>[2x]GSHMNAAAEAEFNILLATDSYKVTHYKQYPPNTSKVYSYFECREKKTENSKVRKVKYEETVFYGLQYILNKYLKGKVVTKEKIQEAKEVYREHFQDDVFNERGWNYILEKYDGHLPIEVKAVPEGSVIPRGNVLFTVENTDPECYWLT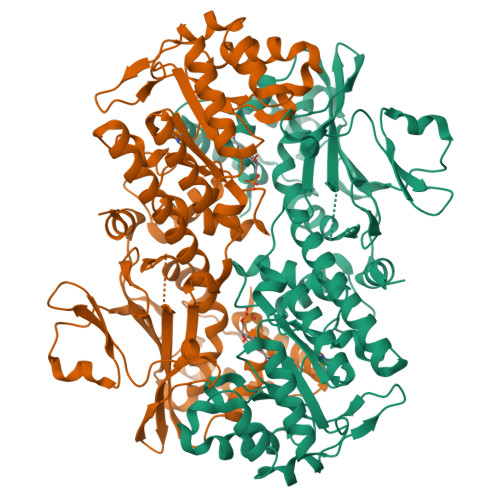NWIETILVQSWYPITVATNSREQKKILAKYLLETSGNLDGLEYKLHDFGYRGVSSQETAGIGASAHLVNFKGTDTVAGIALIKKYYGTKDPVPGYSVPAAEHSTITAWGKDHEKDAFEHIVTQFSSVPVSVVSDSYDIYNACEKIWGEDLRHLIVSRSTEAPLIIRPDSGNPLDTVLKVLDILGKKFPVTENSKGYKLLPPYLRVIQGDGVDINTLQEIVEGMKQKKWSIENVSFGSGGALLQKLTRDLLNCSFKCSYVVTNGLGVNVFKDPVADPNKRSKKGRLSLHRTPAGNFVTLEEGKGDLEEYGHDLLHTVFKNGKVTKSYSFDEVRKNAQLNIEQDVAPH At present, the best structurally characterized pLGIC is the G. violaceus ligand-gated ion channel (GLIC), of prokaryotic origin. Each subunit consists of an extracellular domain (ECD), predominantly in a β-sandwich fold, and a transmembrane domain (TMD) composed of four helices, labeled M1–M4. However, the GLIC is a pH-gated channel, activated by lowering the pH, with a maximal activation at pH 4 and a pH50 around 5. We instead found that proton activation is a complex multiple loci mechanism, with the key contribution stemming from the coupling interface between the extracellular and transmembrane domain, with E35 acting as a key proton-sensing residue.

In contrast to the nonsignificant individual mutations, E26, which is found interacting with the bottom of the β4-β5 loop of the principal (+) face, shows a robust decrease of the pH50 when mutated to both Q and A. A combination of E26Q with mutations of vestibular-facing residues that tend to decrease the pH50 produces an obvious decrease in pH50. A structural analysis was performed on E26Q, E26A, E35Q, E35A, E67A, E75A, E82Q, E82A, D86A, D88N, D88A, H127N, E181A, and H277Q mutants, by solving their structure at pH 4. The key mutants at E26, D86, and D88 were solved at pH 4, each showing a structure similar to that of the Wt. All structures were in the apparently open conformation. E26 clearly is an important residue in GLIC function, but other techniques are required to elucidate its mechanistic role. The report identified E26 and E177 to have loss-of-function effects when mutated. E26 indeed results in a loss-of-function effect, whereas E177 seems to have no effect.

>GQDMVSPPPPIADEPLTVNTGIYLIQCYSLDDKAETFKVNAFLSLSWKDRRLAFDPVRSGVRVKTYEPEAIWIPEIRFVNVENARDADVVDISVSPDGTVQYLERFSARVLSPLDFRRYPFDSQTLHIYLIVRSVDTRNIVLAVDLEKVGKNDDVFLTGWDIESFTAVVKPANFALEDRLESKLDYQLRISRQYFSYIPNIILPMLFILFISWTAFWSTSYEANVTLVVSTLIAHIAFNILVETNLPKTPYMTYTGAIIFMIYLFYFVAVIEVTVQHYLKVESQPARAASITRASRIAFPVVFLLANIILAFLFFGF[5x]alisertib  | C27 H20 Cl F N4 O4 | 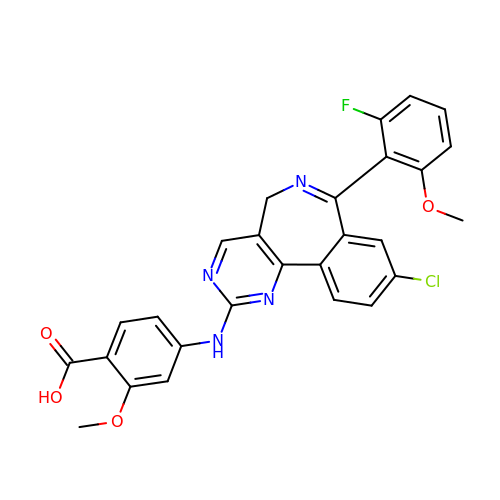ZLHFILGSQDJULK-UHFFFAOYSA-N> SMDAEPGQWDPTLPALVSAGAPGDPLAVANASLQATAQATQTTLDLGRQFLGGLGINLGGPAASAPSAATTGASRIPRANARQAVEYVIRRAGSQMGVPYSWGGGSLQGPSKGVDSGANTVGFDCSGLVRYA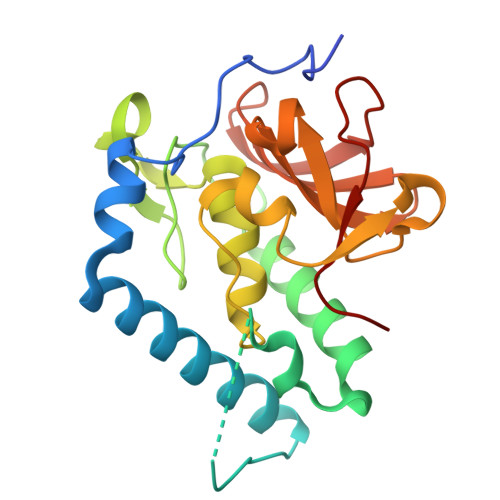FAGVGVLIPRFSGDQYNAGRHVPPAEAKRGDLIFYGPGGGQHVTLYLGNGQMLEASGSAGKVTVSPVRKAGMTPFVTRIIEY> MDCSTNISPKQGLDKAKYFSGKWYVTHFLDKDPQVTDQYCSSFTPRESDGTVKEALYHYNANKKTSFYNIGEGKLESSGLQYTAKYKTVDKKKAVLKEADEKNSYTLTVLEADDSSALVHICLREGSKDLGDLYTVLTHQKDAEPSAKVKSAVTQAGLQLSQF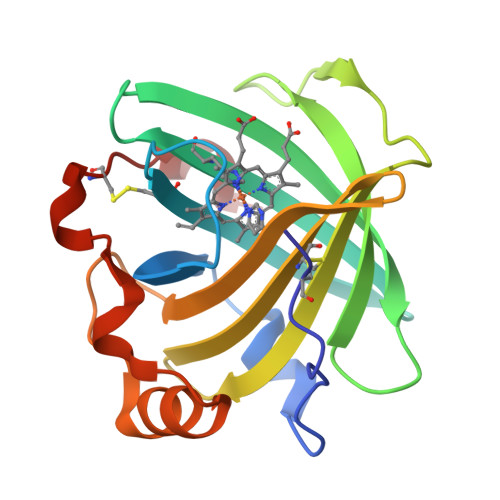VGTKDLGCQYDDQFTSL TrefLec was searched for original domain combinations, which led to single out SaroL-1 in the choanoflagellate Salpingoeca rosetta, that contains both β-trefoil and aerolysin-like pore-forming domains. Recombinant SaroL-1 is shown to bind galactose and derivatives, with a stronger affinity for cancer-related α-galactosylated epitopes such as the glycosphingolipid Gb3, when embedded in giant unilamellar vesicles or cell membranes. SaroL-1 is composed of two domains, a β-trefoil domain at the N-terminal region shown in blue and an elongated domain (green) consisting of seven β-strands forming a twisted β-sheet. The lectin-binding step is necessary for the pore-formation since the pre-incubation with a high affinity galactose derivative diminishes or abolishes hemolysis, GUVs penetration, and cytotoxicity.

The complex of SaroL-1 with the Gb3 trisaccharide presents the same packing as the one with GalNAc. The protein structure is also similar in both complexes albeit with a variation in the fold of the aerolysin β-sheets that present a small kink in its medium region, resulting in an angular deviation of ~17°. The terminal α-galactose of the trisaccharide occupies the exact location and establishes the same contact as GalNAc in the other complex. Electron density was observed in binding sites β and γ only. Site α is not occupied, presumably because of close proximity with the neighboring monomer in the crystal. This packing effect also explains the small kink observed in the aerolysin β-sheet. The second galactose residue (βGal) is perpendicular to His98 in site β and Tyr146 in site γ with hydrogen bonds involving ring oxygen O5 of galactose. In both cases, an acidic amino acid (Asp43 in site β and Glu92 in site γ) bridges between the two Gal residues by establishing two strong hydrogen bonds between O6 of αGal and O2 of βGal. Finally, the reducing Glc also participates in the hydrogen bond network through hydroxyl O2 interacting with Asn42 (site β) or Lys91 (site γ). The location of the terminal αGal is similar in CGL and SaroL-1, while the other part of the trisaccharide shows a significant variation as demonstrated in the superimposition of SaroL-1 and CGL complexes.

>MSSTFEPATDSPLPVPGVQYFLQHVQSGKYVHPHGGSDMPGNDTALVLHHGFDEKRDALRWVFVNDAENKHQLKHYSSGKFVHPKGGKVGKEATLVVHSSPGRPETMIEMVQEDGRTYLRHTDSDYYVHPHGGSPNPGDNTRLVYYSGYRPSLAFLAIPAETLFVDRIEIHQAQALESINTITSLSDEHRNDTDQPVQTSISVALEESLQDSAQLSFERCFGLKVGSEFEVGLPLVGKTKVSVQFSGSWKSSTIKGEVRTSAVKVQINEHVTIPPGKCVQIRIDTRRCTKTAPATMYLRTASGIEVQRETTVTSTYHYDQEVHVVPVTN[2x]> MDAATTRVGLTDLTFRLLRESFADAVSWVAKNLPARPAVPVLSGVLLTGSDNGLTISGFDYEVSAEAQVGAEIVSPGSVLVSGRLLSDITRALPNKPVDVHVEGNRVALTCGNARFSLPTMPVEDYPTLPTLPEETGLLPAELFAEAISQVAIAAGRDDTLPMLTGIRVEILGETVVLAATDRFRLAVRELKWSASSPDIEAAVLVPAKTLAEAAKAGIGGSDVRLSLGTGPGVGKDGLLGISGNGKRSTTRLLDAEFPKFRQLLPTEHTAVATMDVAELIEAIKLVALVADRGAQVRMEFADGSVRLSAGADDVGRAEEDLVVDYAGEP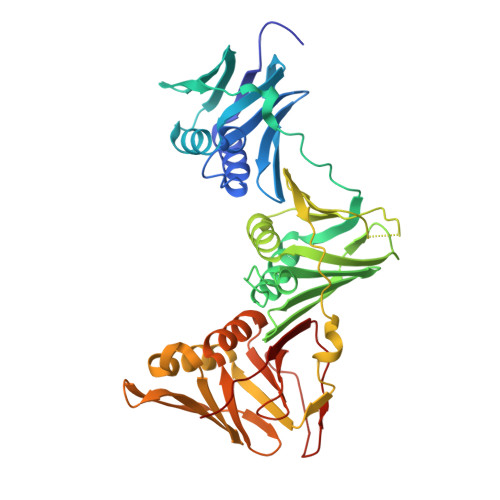LTIAFNPTYLTDGLSSLRSERVSFGFTTAGKSALLRPVSGDDRPVAGLNGNGPFPAVSTDYVYLLMPVRLPG> GAMGKSEGVTIEFKIVGLNKKLKVFTTCPHTLFGASFCAVAIEHPIVQDLMSKEIQDLISSIKIQGKNNEKVGIYTGLNVKHPFLDKELPLYVANFVLMEYREGAIFGCPAHDQRDFEFAQEYDLPIIPVISSARLGIEEYTNNSIMFNSEFLNGLTVSEARKVIVEKLEEKGIGKKTI

Here, we report the discovery of potent boron-based compounds that inhibit an unprecedented target of Wolbachia, leucyl-tRNA synthetase (LeuRS), and demonstrate that inhibition of this microbiota target is an efficient approach to arrest the growth of its host. The editing site of LeuRS plays a key role to maintain fidelity in protein translation by hydrolyzing tRNALeu mischarged to noncognate amino acids such as norvaline. Altogether, these experiments show that benzoxaborole inhibitors of Wolbachia LeuRS are prodrugs that, in an enzyme-independent manner, form adducts with adenosine substrates. The adducts then bind with potent nanomolar affinity into the Wolbachia LeuRS editing site and efficiently compete with the physiological substrate norvaline.

(A) Overall structure of the Wolbachia LeuRS complex with the adduct AMP-Cmpd6 bound into the editing site. In the absence of AMP, Cmpd6 and Cmpd9 did not bind to Wolbachia LeuRS; however, in the presence of AMP, the compounds were potent LeuRS inhibitors, with dissociation constants of 44 and 6 nM, respectively. The potent nanomolar affinities of the two compounds are explained by a combination of multiple polar and hydrophobic interactions established by the inhibition adducts in the editing site. Both compounds make equivalent interactions with Wolbachia LeuRS, except for minor differences in the 2-amido-thiazole and amino-methyl phenyl groups of Cmpd6 and Cmpd9, respectively. In Cmpd6, the 2-amido-thiazole group enables multiple polar contacts to the side chains of R330 and Y316, the latter further being stabilized by interactions of the adenosine-phosphate with Y316 and R317 and an intramolecular interaction within Cmpd6 established by the sulfur atom with the neighboring carbonyl. Furthermore, the oxygen at position 7 hydrogen bonds to the side chain of R330. The amido-thiazole group also packs against the adenosine ring; however, the π-π stacking is not entirely parallel compared to the phenyl of Cmpd9. Other key interactions, shared by the two compounds, are a hydrogen bond by the oxaborole oxygen-1 to T241; and the three hydrogen bonds established by the 3-aminomethyl to F322, D328, and D331. In the adduct formed with AMP, the phenyl and amido-thiazole groups stack against the adenosine base and enable multiple interactions within the Wolbachia LeuRS drug pocket.> IVGGT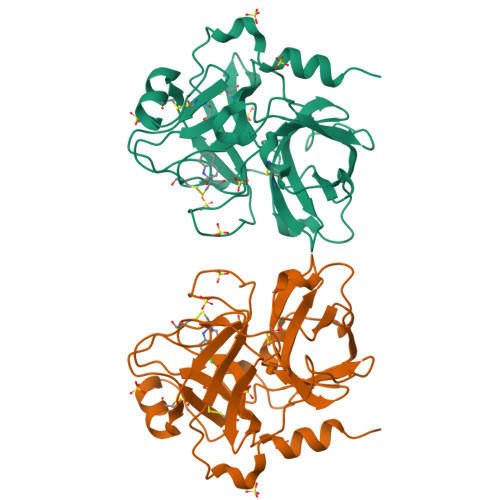ASVRGEWPWQVTLHTTSPTQRHLCGGSIIGNQWILTAAHCFYGVESPKILRVYSGILNQAEIAEDTSFFGVQEIIIHDQYKMAESGYDIALLKLETTVNYADSQRPISLPSKGDRNVIYTDCWVTGWGYRKLRDKIQNTLQKAKIPLVTNEECQKRYRGHKITHKMICAGYREGGKDACKGDSGGPLSCKHNEVWHLVGITSWGEGCAQRERPGVYTNVVEYVDWILEKTQAV> PVTTSFWRIATDARTYEADDL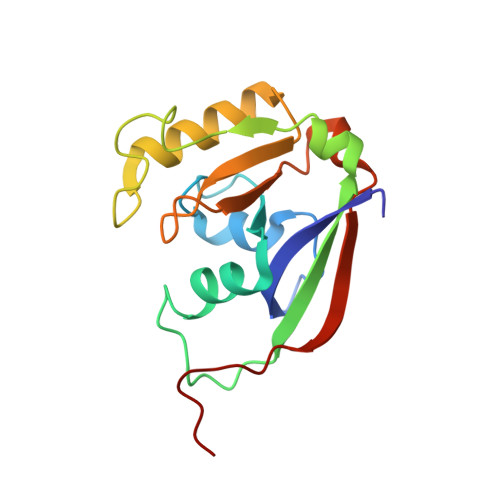SGAGAKITGGRWNEVGVAIVYAASSRALACLETVVHLNSGGLPLNRYLVEIEVPDEVLASAEVATPGNLPVGWDAEPAGRVSISFGSQWAQSQRTALLLVPSVIVPEETNLLINPAHPDAKGIKARKVRKWLYDPRMIR> GSHMASMLPEETILDKLPKDFQERITSSKWKDRVEALEEFWDSVLSQTKKLKSTSQNYSNLLGIYGHIIQKDANIQAVALAAQSVELICDKLKTPGFSKDYVSLVFTPLLDRTKEKKPSVIEAIRKALLTICKYYDPLASSGRNEDMLKDILEHMKHKTPQIRMECTQLFNA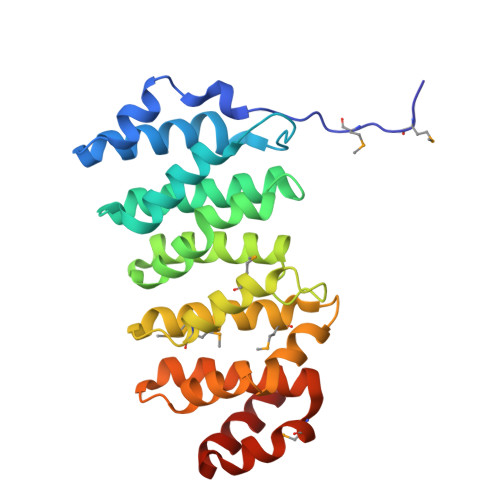SMKEEKDGYSTLQRYLKDEVVPIVIQIVNDTQPAIRTIGFESFAILIKIFGMNTFVKTLEHLDNLKRKKIEETVKTL>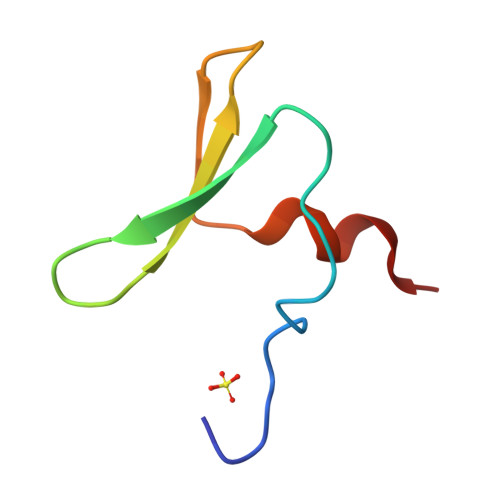 GAMGFEIPDDVPLPAGWEMAKTSSGQRYFLNHIDQTTTWQDPRKAMLSQ>[3x]MGRVRLVQFQKNTDEPMGITLKMNELNHCIV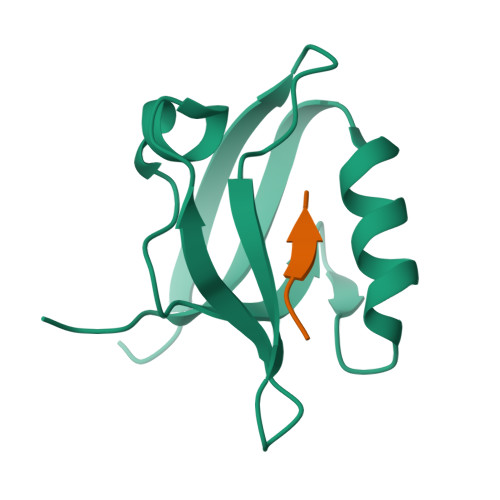ARIMHGGMIHRQGTLHVGDEIREINGISVANQTVEQLQKMLREMRGSITFKIVPSYR;>KKNKDKEYYV[3x]>[2x]MSLLERGLSKLTLNAWKDREGKIPAGSMSAMYNPETIQLDYQTRFDTEDTINTASQSNRYVISEPVGLNLTLLFDSQMPGNTTPIETQLAMLKSLCAVDAATGSPYFLRITWGKMRWENKGWFAGRARDLSVTYTLFDRDATPLRATVQLSLVADESFVIQQSLKTQSAPDRALVSVPDLASLPLLALSAGGVLASSVDYLSLAWDNDLDNLDDFQTGDFLRATKGEEV;> MSHITLDIAGQRSTLGIRRLRVQQLINEIPLAQLELHIPTDNHGAADNAVQHEVSRFTLGVRVGIAQDNKPLFDGYLVQKKMQLKGKEWSVRLEARHALQKLTFLPHSRVFRQQDDSTVMKGLLQSAGVKLTQESAAQLSSKHDQLLQFRLSDWQFIRSRLLSTNCWLLPDAASDTVVIRPLSDAAMASRTLARDSHDYTLYEINLNFDNRFTPDSLSLQGWDIAAQRLTAAQKSPAGAFRPWKPAGKVGQSSAGRQDYALAFSMLPEATLQTL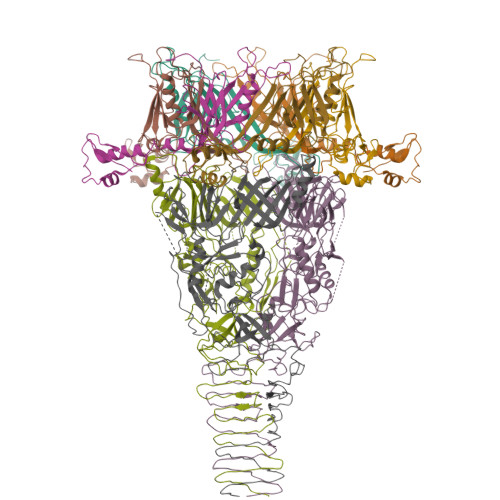SNSWLNYQQMTGVQGHIVLAGTRDFAPGESITLSGFGAGLDGTAMLSGVNQQFDTQYGWRSELVIGLPASMLEPAPPVRSLHIGTVAGFTADPQHLDRIAIHLPALNLPDSLIFARLSKPWASHASGFCFYPEPGDEVVVGFIDSDPRYPMILGALHNPKNTAPFPPDEKNNRKGLIVSQADQTQALMIDTEEKTLRLMAGDNTLTLTGEGNLTMSTPNALQLQADTLGLQADSNLSIAGKQQVEITSAKINMKK> STILVIHGPNLNLLGKREPEVYGHLTLDNINRQLIAQAEQASITLDTFQSNWEGAIVDRIHQAQTEGVKLIIINPA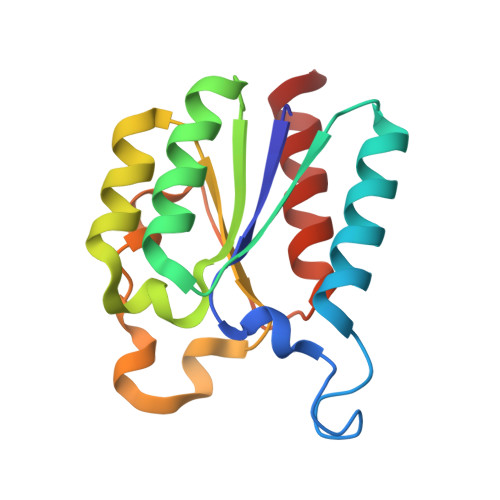ALTHTSVALRDALLGVAIPFIEVHLSNVHAREAFRHHSYLSDKAIGVICGLGAKGYSFALDYAIEKIQP>MDTNKREIVEFLGIRTYFFPNLALYAVNNDELLVSDPNKANSFAAYVFGASDKKPSVDDIVQILFPSGSDSGTILTSMDTLLALGPDFLTEFKKRNQDLARFNLTHDLSILAQGDEDAAKKKLNLMGRKAKLQKTEAAKILAILIKTINSEENYEKFTELSELCGLDLDFDAYVFTKILGLED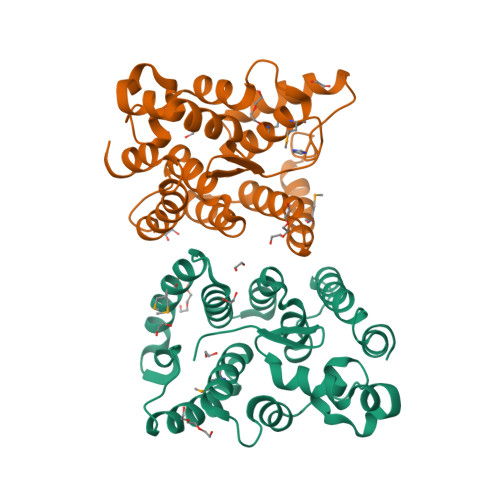EDTADEVEVIRDNFLNRLDQTKPKLADIIRNGP[4x]> QRDLSVELGVASNFAILAKAGISSVPDSAILGDIGVSPAAATYITGFGLTQDSSTTYATSPQVTGLIYAADYSTPTPNYLAAAVANAETAYNQAAGFVDPDFLELGAGELRDQTLVPGLYKWTSSVSVPTD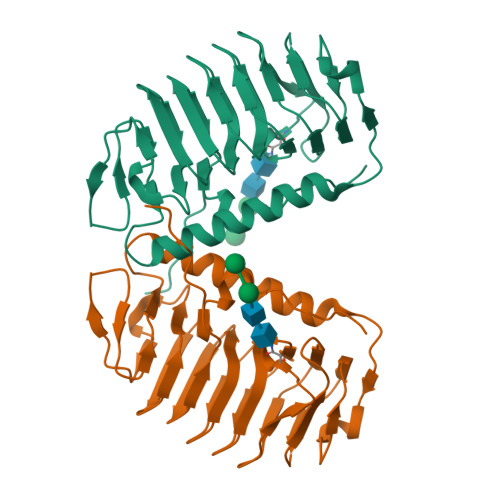LTFEGNGDATWVFQIAGGLSLADGVAFTLAGGANSTNIAFQVGDDVTVGKGAHFEGVLLAKRFVTLQTGSSLNGRVLSQTEVALQKATVNSPFVPAPEVVQKRSNARQWL> GPHMRYSKVDLLALRYEGKSRQRPQCSTRL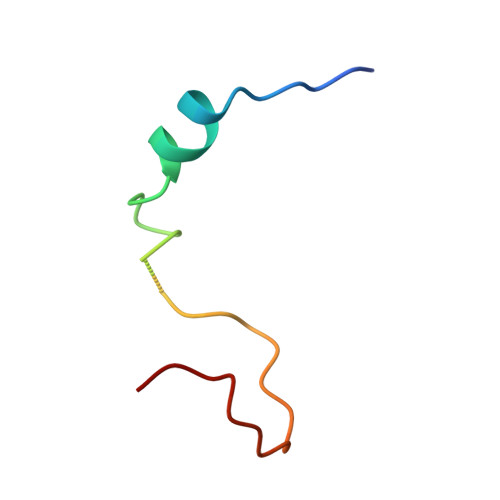ELQTLGFWKI> GTQSTHESLKPQRVQFQSRN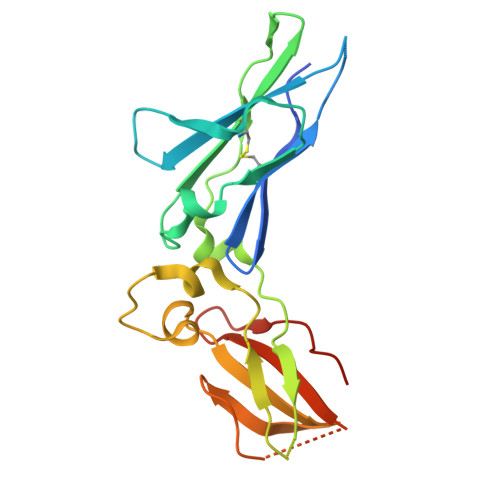FHNILQWQPGRALTGNSSVYFVQYKIYGQRQWKNKEDCWGTQELSCDLTSETSDIQEPYYGRVRAASAGSYSEWSMTPRFTPWWETKIDPPVMNITQVNGSLLVILHAPNLPYRYQKEKNVSIEDYYELLYRVFIINNSLEKEQKVYEGAHRAVEIEALTPHSSYCVVAEIYQPMLDRRSQRSEERCVEIP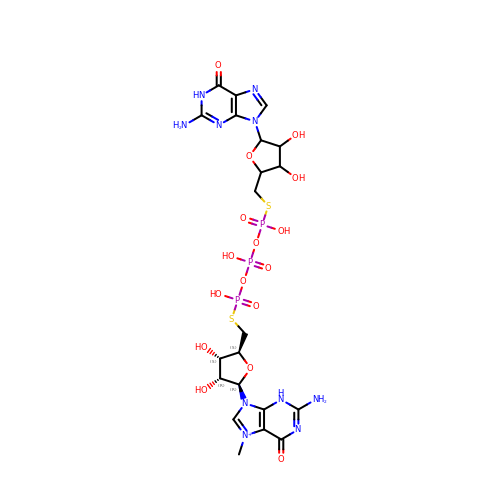[(2~{S},3~{S},4~{R},5~{R})-5-(2-azanyl-7-methyl-6-oxidanylidene-3~{H}-purin-7-ium-9-yl)-3,4-bis(oxidanyl)oxolan-2-yl]methylsulfanyl-[[[(3~{R},4~{S})-5-(2-azanyl-6-oxidanylidene-1~{H}-purin-9-yl)-3,4-bis(oxidanyl)oxolan-2-yl]methylsulfanyl-oxidanyl-phosphoryl]oxy-oxidanyl-phosphoryl]oxy-phosphinic acid | C21 H30 N10 O16 P3 S2 | YZDSTSNLJBCGKH-KVTZQEPKSA-O>MNHKVHHHHHHIEGRHMKVNISIFGFGTVGRALAEIIAEKSRIFGVELNVISITDRSGTIWGDFDLLEAKEVAESTGKLSNIGDYEVYNFSPQELVEEVKPNILVDVSSWDEAHEMYKVALGEGISVVTSNKPPIANYYDELMNLAKENNAGIFFESTVMAGTPIIGVLRENLLGENIKRIDAVVNASTTFILTKMSEGKTLDDAIEEAKSLGILEEDPSKDIDGIDAYYKAKILHWVSYGEPPEEEERLGIREVRDARNVRLVAQVSKGKISVKPRKLSSDNPLLVEGVQNAAVIRTNNLGEVILKGPGGGGRVTASGVFTDIIKATLKFPNLR[2x]

Homoserine dehydrogenase (HseDH, EC 1.1.1.3) is a key enzyme in the biosynthetic pathway from aspartate to homoserine (Hse), which is a common precursor for the synthesis of three amino acids, methionine, threonine and isoleucine in plants and microorganisms. The third enzyme in the pathway, HseDH, catalyzes the NAD(P)H-dependent reduction of Asa to Hse. In the present study, we expressed that gene, which encoded a HseDH homolog, characterized the enzyme produced and revealed the enzyme to be a highly thermostable HseDH. Each monomer consisted of three domains: a nucleotide-binding domain (residues 1–139 and 297–315), a dimerization domain (140–160 and 266–293) and a substrate-binding domain (residues 161–265).

To reduce the number of these interactions, we constructed R40A and K57A mutants, which had striking effects on the enzymes reactivity against NADP. The model of the Hse-bound K57A mutant was refined at a resolution of 2.43 Å. The model of the dimer contained the ordered residues (1–319) in each subunit, two NADPH molecules, two Hse molecules, two Na atoms and 211 water molecules. Moreover, we also observed an extra density within the active site cavity, and after construction and refinement of the peptide chain, a Hse molecule could be modeled into that density. Within our model, the carboxyl group of Hse hydrogen bonded with the side-chain of Asp206 and the backbone N atoms of Ala171 and Ser172 and, via a water molecule (W5), with the backbone O atom of Ile198. The O atom of the C4 hydroxyl group interacts with the side-chains of Lys116 and Lys215 and, via another water molecule (W6), with the backbone N atoms of Met144 and Ala145 and the backbone O atom of Gly294. The C4 atom of Hse is situated in front of the C4 atom of the nicotinamide ring, which enables hydride transfer between the two. Superposition of the Hse/NADPH-bound K57A structure onto the NADPH-bound wild-type structure showed that the NADPH molecule in the mutant structure was positioned/configured nearly identically to the NADPH molecule in the wild-type structure, except for the positioning of the C2 phosphate group of the adenine ribose. In K57A mutant, however, the C2 phosphate group is rotated in a clockwise direction around C2B of NADPH by about 30° relative to the wild-type structure. In addition, the guanidino group of Arg40 in the mutant is also rotated clockwise by about 90° around the NE atom of Arg40 relative to the wild-type structure.>AIPSSLSINWNNYATGAYSSGNAASDFGNAGGWNQSRSYISDGTLRVTLLKNALSGAGGLISNIDVSDGTEYELDYDVRFHSQFDWSRGGAVGFGFSIGEGNTGGDPGWDGNGGTLRMMWYQTDAGRVFFQPAIYHKDQPGQYGDTFGKSYPSS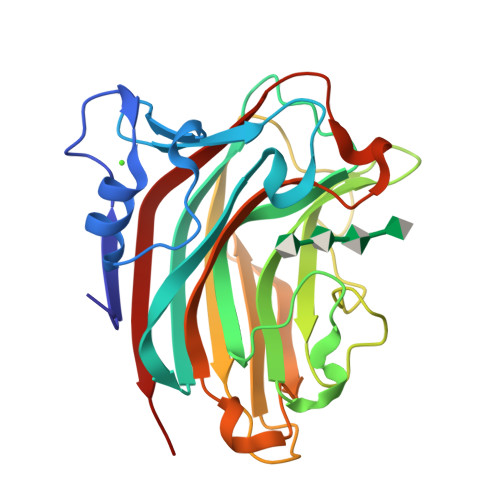GSITKGTTYHVHVYIKSNTGSNRDGRAQIIINGTTVLDTAIRWTTNDAQRLIKNMTFHTFRGGSQTYWQSPVDSYIYYDNLVLRKIRLEH[3x]>GPGSMAIEEILDLEQLEVNIYRGSVFSPESGFLQRTFGGHVAGQSLVSAVRTVDPRYQVHSLHGYFLRSGDAQEPTVFLVERTRDGGSFVTRRVNAVQHGEVIFSMGASFQTAQNGISHQDAMPAAPPPDDLPGLRSVRVFDDAGFRQFEEWDVRIVPRDLLAPLPGKASQQQVWFRHRDPLPDDPVLHICALAYMSDLTLLGSAQVTHLAEREHLQVASLDHAMW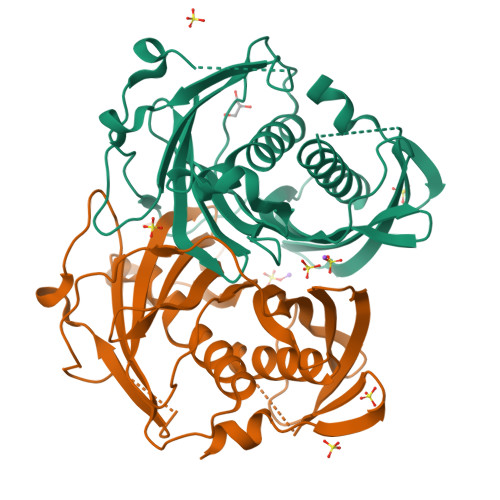FMRGFRADEWLLYDQSSPSAGGGRALTHGKIFTQGGELVAAVMQEGLTRYPSGYQPGEK[2x]tert-butyl (2S)-3-[4-amino-7-(3-hydroxypropyl)-5-(4-methylphenyl)-7H-pyrrolo[2,3-d]pyrimidin-6-yl]-2-cyanopropanoate 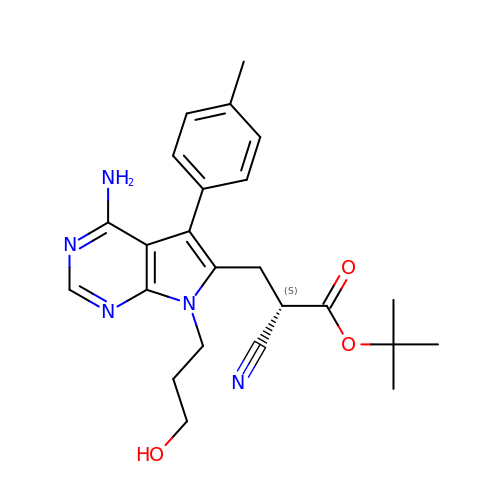| C24 H29 N5 O3 | YQNJEMHLWSEPFO-KRWDZBQOSA-N>[3x]DRLGQPPSGYGVLLSVHEDKTVDVFTSGRKMRLTCSPNIDTDTLALGQTVRLNEALTIVEAGTYEQVGEIST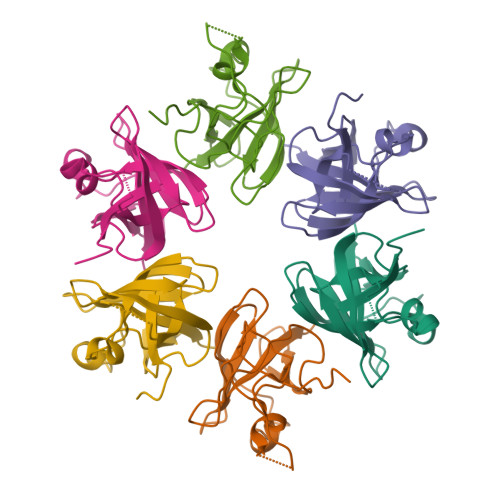LREVLDDGLRALVVGHADEERIVWLAAPLAAVFADPEADIIAYDADSPTRKLRPGDSLLVDTKAGYAFERIPKAEVEDLVL> PCIEVVPNITYQCMDQKLSKVPDDIPSSTKNIDLSFNPLKILKSYSFSNFSELQWLDLSRCEIETIEDKAWHGLHHLSNLILTGNPIQSFSPGSFSGLTSLENLVAVETKLASLESFPIGQLITLKKLNVAHNFIHSCKLPAYFSNLTNLVHVDLSYNYIQTITVNDLQFLRENPQVNLSLDMSLNPIDFIQDQA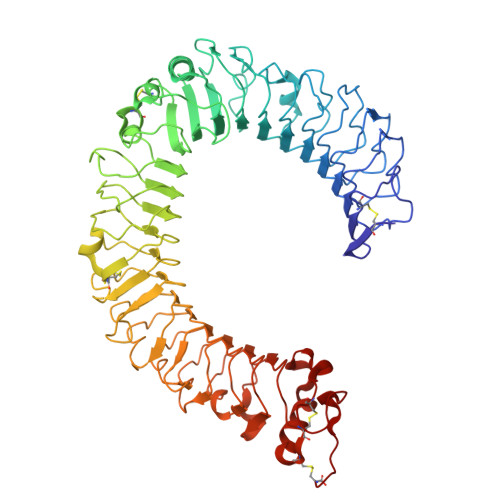FQGIKLHELTLRGNFNSSNIMKTCLQNLAGLHVHRLILGEFKDERNLEIFEPSIMEGLCDVTIDEFRLTYTNDFSDDIVKFHCLANVSAMSLAGVSIKYLEDVPKHFKWQSLSIIRCQLKQFPTLDLPFLKSLTLTMNKGSISFKKVALPSLSYLDLSRNALSFSGCCSYSDLGTNSLRHLDLSFNGAIIMSANFMGLEELQHLDFQHSTLKRVTEFSAFLSLEKLLYLDISYTNTKIDFDGIFLGLTSLNTLKMAGNSFKDNTLSNVFANTTNLTFLDLSKCQLEQISWGVFDTLHRLQLLNMSHNNLLFLDSSHYNQLYSLSTLDCSFNRIETSKGILQHFPKSLAFFNLTNNSVACICEHQKFLQWVKEQKQFLVNVEQMTCATPVEMNTSLVLDFNNSTC> SNAANDAGKSDLDAAVEATIPPLMKAKDIPGMAVAVLADGKAHYFNYGVASRETGQPVTQDTLFELGSISKTFTGILGGYALAQGKLSLADKASRYQPELKGSVFDRVSLLQLATYSAGGLPLQFPDAVAGQASMLAYYRGWKPDYAPGERRLYSNPSIGLFGHLAARSLGQPFDQAMERGLLPKLGLSHTFIHVPEAEQSRYAWGYAKAGKPIRVGAGVLDAEAYGIKSSAADLLKYLAINMSPPADPALQRALDASHAAYYRVGDMRQGLGWEGYRYPISLERLLAGNSNEIAFQPQKVEWLNPPRLAEGDVLLNKTGSTSGFGAYVLFVPARKVGIVMLANRNYPN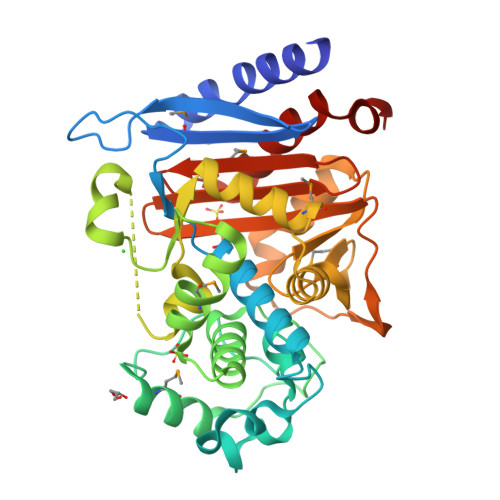AERVRAAYRILSAVDPSLVRRRGD>[2x]GPLGSSLHIYNWTDYIAPTTLKDFTKESGIDVSYDVFDSNETLEGKLVSGHSGYDIVVPSNNFLGKQIQAGAFQKLDKSKLPNWKNLDPALLKQLEVSDPGNQYAVPYLWGTNGIGYNVAKVKEVLGDQPIDSWAILFEPENMKKLAKCGVAFMDSGDEMLPAALNYLGLDPNTH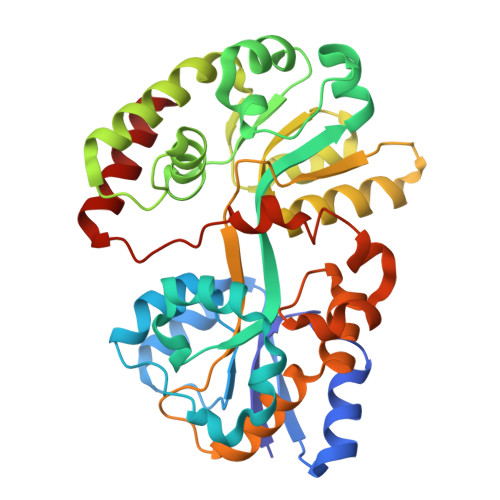DPKDYKKAEEVLTKVRPYVSYFHSSKYISDLANGNICVAFGYSGDVFQAAARAEEAGKGIDIQYVIPKEGANLWFDLMAIPADAKAADNAYAFIDYLLRPEVIAKVSDYVGYANAIPGARPLMDKSVSDSEEVYPPQAVLDKLYVSAVLPAKVLRLQTRTWTRIK>[4x]FQKIYSPTQLANAMKLVRQQNGWTQS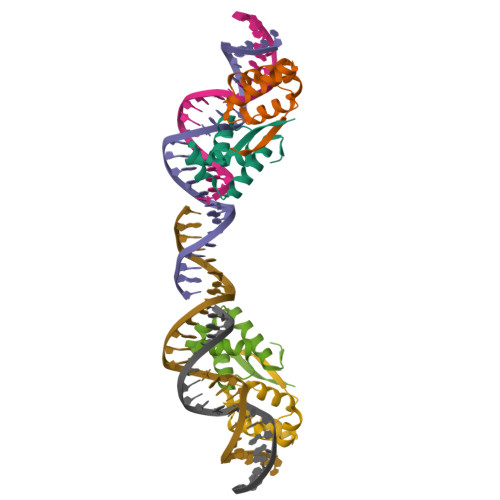ELAKKIGIKQATISNFENNPDNTTLTTFFKILQSLELSMTLCDAK>MLGAVEGPRWKQAEDIRDIYDFRDVLGTGAFSEVILAEDKRTQKLVAIKCIAKEALEGKEGSMENEIAVLHKIKHPNIVALDDIYESGGHLYLIMQLVSGGELFDRIVEKGFYTERDASRLIFQVLDAVKYLHDLGIVHRDLKPENLLYYSLDEDSKIMISDFGLSKMEDPGSVLSTACGTPGYVAPEVLAQKPYSKAVDCWSIGVIAYILLCGYPPFYDENDAKLFEQILKAEYEFDSPYWDDISDSAKDFIRHLMEKDPEKRFTCEQALQHPWIAGDTALDKNIHQSVSEQIKKNFAKSKWK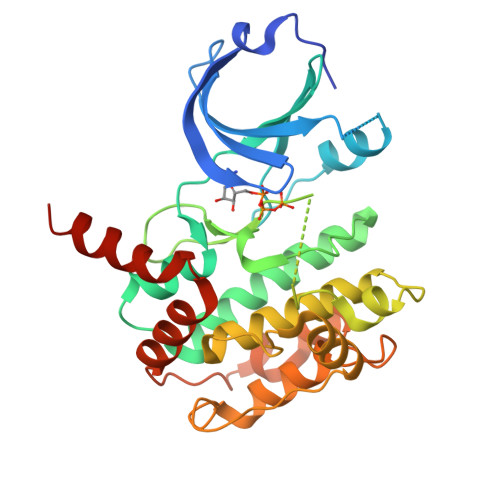QAFNATAVVRHMRKLQ[2x]>MNIRERKRKHLEACLEGEVAYQKTTTGLEGFRLRYQALAGLALSEVDLTTPFLGKTLKAPFLIGAMTGGEENGERINLALAEAAEALGVGMMLGSGRILLERPEALRSFRVRKVAPKALLIANLGLAQLRRYGRDDLLRLVEMLEADALAFHVNPLQEAVQRGDTDFRGLVERLAELLPLPFPVMVKEVGHGLSREAALALRDLPLAAVDVAGAGGTSWARVEEWVRFGEVRHPELCEIGIPTARAILEVREVLPHLPLVASGGVYTGTDGAKALALGADLLAVARPLLRPALEGAERVAAWIGDYLEEL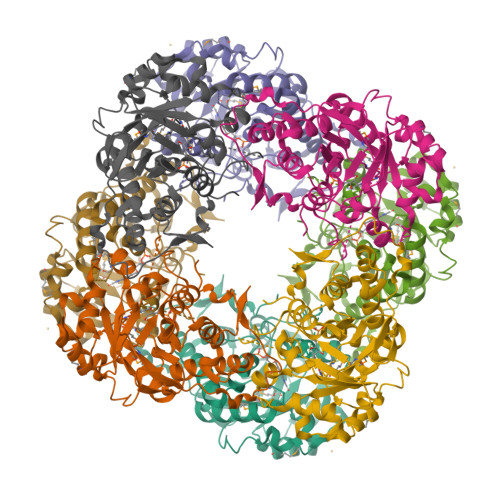RTALFAIGARNPKEARGRVERV[2x]>LGNY[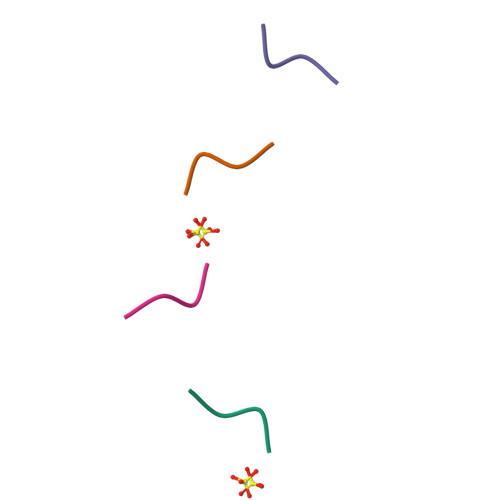4x]> MGSDKIHHHHHHMNDLVESLIYEVNNMQQNFENVKSQQQDHDFYQTVKPYTEHIDSILNEIKLHREFIIEVPYMNSRKFELLIANIEQLSVECHFKRTSRKLFIEKLKSVQYDLQNIL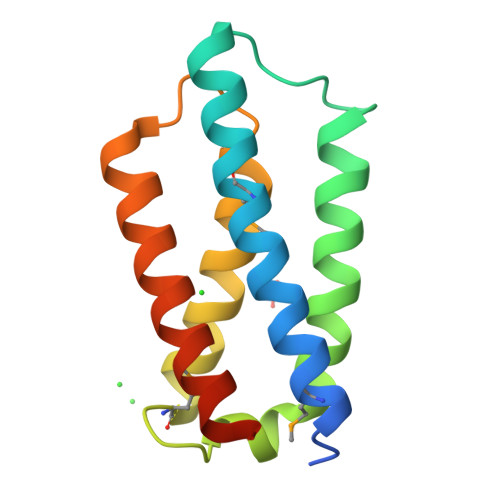DGVTKEGTDG> 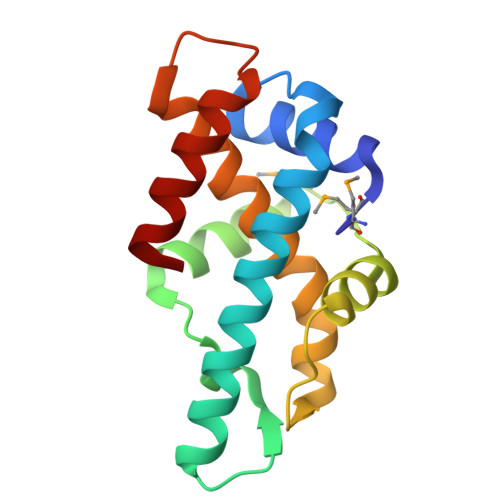MLMKVAEFERLFRQAAGLDVDKNDLKRVSDFLRNKLYDLLAVAERNAKYNGRDLIFEPDLPIAKGLQETLQEFRRMDTALELKPVLDALAALPPLDLEVAEDVRNLLPELAGALVVAYARVLKELDPALKNPQTEHHERAERVFNLLL>MNAAAEAEFNILLATDSYKVTHYKQYPPNTSKVYSYFECREKKTENSKVRKVKYEETVFYGLQYILNKYLKGKVVTKEKIQEAKEVYREHFQDDVFNERGWNYILEKYDGHLPIEVKAVPEGSVIPRGNVLFTVENTDPECYWLTNWIETILVQSWYPITVATNSREQKKILAKYLLETSGNLDGLEYKLHDFGYRGVSSQETAGIGAS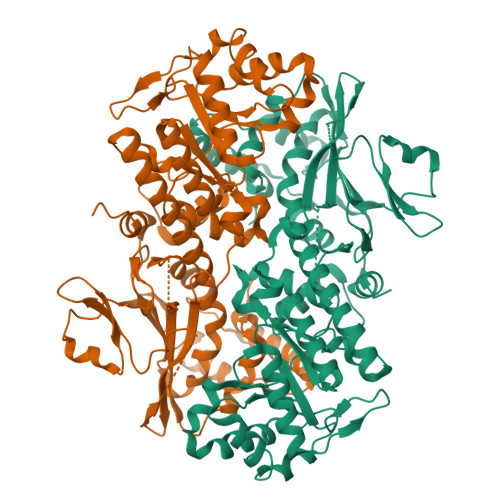AHLVNFKGTDTVAGIALIKKYYGTKDPVPGYSVPAAEHSTITAWGKDHEKDAFEHIVTQFSSVPVSVVSDSYDIYNACEKIWGEDLRHLIVSRSTEAPLIIRPDSGNPLDTVLKVLDILGKKFPVSENSKGYKLLPPYLRVIQGDGVDINTLQEIVEGMKQKKWSIENVSFGSGGALLQKLTRDLLNCSFKCSYVVTNGLGVNVFKDPVADPNKRSKKGRLSLHRTPAGTFVTLEEGKGDLEEYGHDLLHTVFKNGKVTKSYSFDEVRKNAQLNMEQDVAPH[2x]>[2x]MATVAVVPAAGSGERLRAGRPKAFVTLGGTPLLEHALSGLRASGVIDRIVIAVPPALTDESKLVFGGEDSVIVSGGVDRTESVALALEA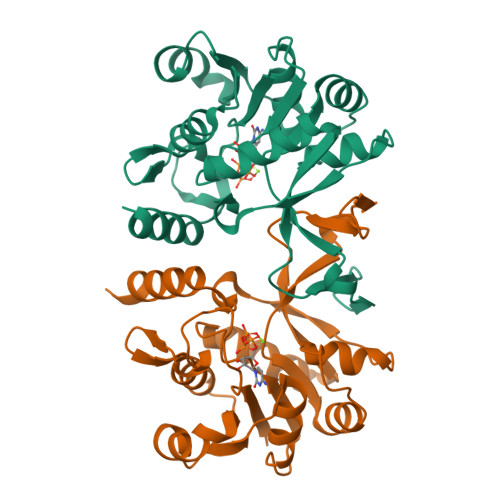AGDAEFVLVHDAARALTPPALIARVVAALKEGHSAVVPGLAPADTIKAVDANGAVLGTPERAGLRAVQTPQGFHADVLRRAYARATAGGVTDDASLVEQLGTPVQIVDGDPLAFKITTPLDLVLAEAVLAHHHH>[4x]MSKLIVPQWPQPKGVAACSSTRIGGVSLPPYDSLNLGAHCGDNPDHVEENRKRLFAAGNLPSKPVWLEQVHGKDVLKLTGEPYASKRADASYSNTPGTVCAVMTADALPVLFCNRAGTEVAAAHAGWRGLCAGVLEETVSCFADNPENILAWLGPAIGPRAFEVGGEVREAFMAVDAKASAAFIQHGDKYLADIYQLARQRLANVGVEQIFGGDRCTYTENETFFSYRRDKTTGRMASFIWLILEHH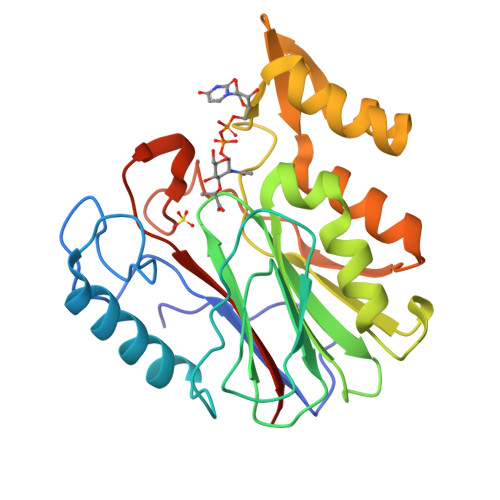HHHH> GSGEGPREPGAAGGAAGGSRDALSLEEILRLYNQPIN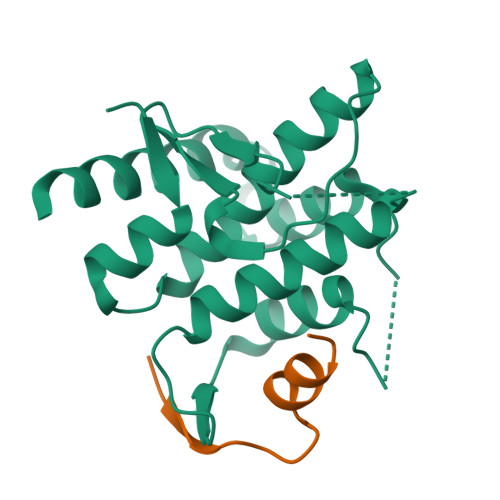EEQAWAVCYQCCGSLRAAARRRQPRHRVRSAAQIRVWRDGAVTLAPAADDAGEPPPVAGKLGYSQCMETEVIESLGIIIYKALDYGLKENEERELSPPLEQLIDHMANTVEADGSNDEGYEAAEEGLGDEDEKRKISAIRSYRDVMKLCAAHLPTESDAPNHYQAVCRALFAETMELHTFLTK;> KSLYKIKPRHDSGIKAKISMKT>MSSGNAKIGHPAPNFKATAVMPDGQFKDISLSDYKGKYVVFFFYPLDFTFVSPTEIIAFSDRAEEFKKLNCQVIGASVDSHFSHLAWVNTPKKQGGLGPMNIPLVSDPKRTIAQDYGVLKADEGISF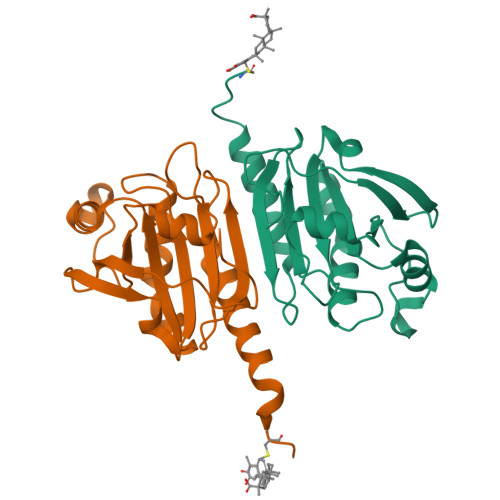RGLFIIDDKGILRQITVNDLPVGRSVDETLRLVQAFQFTDKHGEVCPA[2x]>[4x]MRLEPEIKEFRQERKTLQLATVDAQGRPNVSYA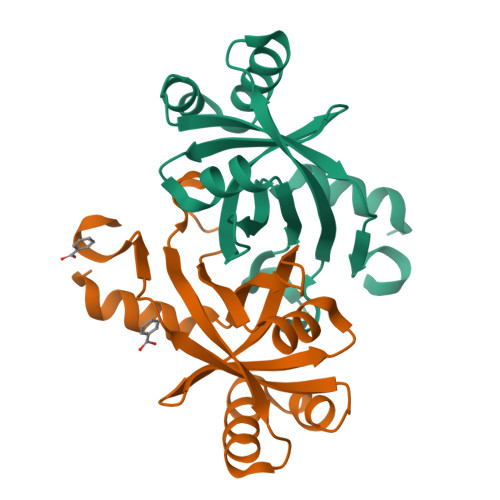PFVQNQEGYFVLISHIARHARNLEVNPQVSIMMIEDETEAKQLFARKRLTFDAVASMVERDSELWCQVIAQMGERFGEIIDGLSQLQDFMLFRLQPEQGLFVKGFGLEHHHHHHH> GAADPVVVPANMEPLTIEGNRFVTLCIMIRTTPWEVSRDVKLHPRDEVDWHTLEGVRALREAFATNNPNGRLTWGFTMNALEDGRKNYREIRDYVVECQKKYGDEVTYFPGYFPAMYLPRERVNREMSEAIEIISKMVGNGYRPQSIMGGFLSADNLRYLAEKENIHVAHAVIWSQHNIDGGGADGSPSYPFYPSTEHFCKPAQGKSDFIDCVNLDGWTMDFICARRSGQTGHGIDGYNSRRGVGPIETYKGWGLDLGHREVMHTEAIHFDKGLELNGFGWVANIWEAQMVHEFGKDLICDAMKMWVTGTKERWPDTHF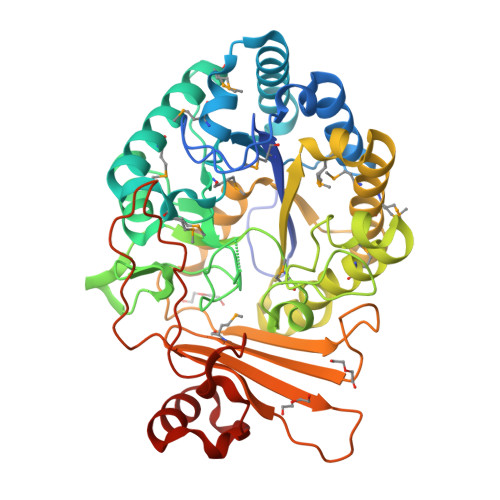VTFGEFGELWRKQYKSNDDWNYRFVERGSGLGDSYNNLEIKWFMNKEFRLALLRDWHTKNSPAYVIDFTRYDLQAHEPADPSPEKPAKDWSLINKINQKALRPQDKPVLIDKLEKEDQDLIRKYYPELLK> HIEGYECQPIFLNVLEAIEPGVVCAGHDNNQPDSFAALLSSLNELGERQLVHVVKWAKALPGFRNLHVDDQMAVIQYSWMGLMVFAMGWRSFTNVNSRMLYFAPDLVFNEYRMHKSRMYSQCVRMRHLSQEFGWLQITPQEFLCMKALLLFSIIPVDGLKNQKFFDELRMNYIKELDRIIACKRKNPTSCSRRFYQLTKLLDSVQPIARELHQFTFDLLIKSHMVSVDFPEMMAEIISVQ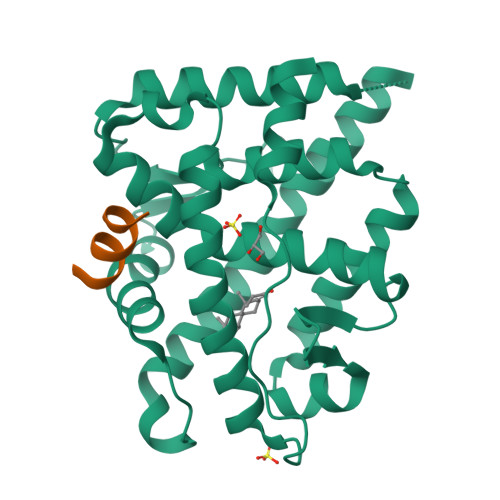VPKILSGKVKPIYFHTQ;> RGAFQNLFQSV>[8x]THPDISVDVLVIGAGPTGLGAAKRLNQIDGPSWMIVDSNETPGGLASTDVTPEGFLYDVGGHVIFSHYKYFDDCLDEALPKEDDWYTHQRISYVRCQGQWVPYPFQNNISMLPKEEQVKCIDGMIDAALEARVANTKPKTFDEWIVRMMGTGIADLFMRPYNFKVWAVPTTKMQCAWLGERVAAPNLKAVTTNVILGKTAGNWGPNATFRFPARGGTGGIWIAVANTLPKEKTRFGEKGKVTKVNANNKTVTLQDGTTIGYKKLVSTMAVDFLAEAMNDQELVGLTKQLFYSSTHVIGVGVRGSRPERIGDKCWLYFPEDNCPFYAATIFSNYSPYNQPEASKKLPTMQLADGSRPQSTEAKEGPYWSIMLEVSESSMKPVNQETILADCIQGLVNTEMLKPTDEIVSTYHRRFDHGYPTPTLEREGALTQILPKLQDKDIWSRGRFGSWRYEVGNQDHSFMLGVEAVDNIVNGAVELTLNYPDFVNGRQNTERRLVDGAQVFA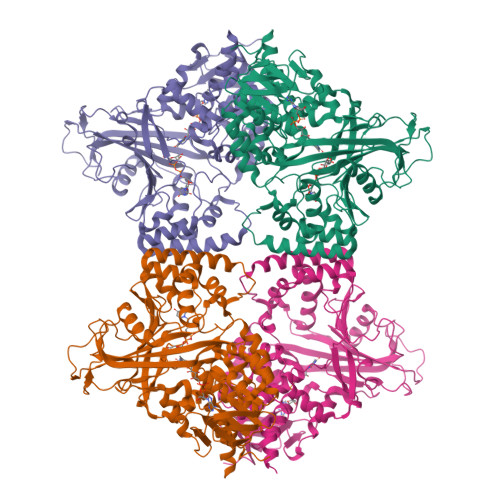KSKAQ> GSHMASADNNSAIYFNTSQPINDLQGSLAAEVKFAQSQILPAHPKEGDSQPHLTSLRKSLLLVRPVKADDKTPVQVEARDDNNKILGTLTLYPPSSLPDTIYHLDGVPEGGIDFTPHNGTKKIINTVAEVNKLSDASGSSIHSHLTNNALVEIHTANGRWVRDIYLPQGPDLEGKMVRFVSSAGYSSTVFYGDRKVTLSVGNTLL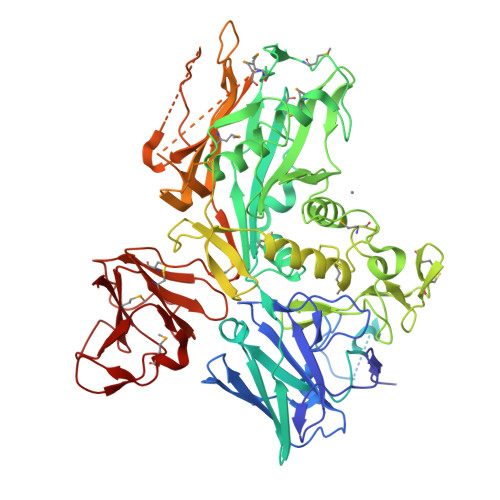FKYVNGQWFRSGELENNRITYAQHIWSAELPAHWIVPGLNLVIKQGNLSGRLNDIKIGAPGELLLHTIDIGMLTTPRDRFDFAADAAAHREYFQTIPVSRMIVNNYAPLHLKEVMLPTGELLTDMDPGNGGWHSGTMRQRIGKELVSHGIDNANYGLNSTAGLGENSHPYVVAQLAAHNSRGNYANGIQVHGGSGGGGIVTLDSTLGNEFSHDVGHNYGLGHYVDGFKGSVHRSAENNNSTWGWDGDKKRFIPNFYPSQTNEKSCLNNQCQEPFDGHKFGFDAMAGGSPFSAANRFTMYTPNSSAIIQRFFENKAVFDSRSSTGFSKWNADTQEMEPYEHTIDRAEQITASVNELSESKMAELMAEYAVVKVHMWNGNWTRNIYIPTASADNRGSILTINHEAGYNSYLFINGDEKVVSQGYKKSFVSDGQFWKERDVVDTREARKPEQFGVPVTTLVGYYDPEGTLSSYIYPAMYGAYGFTYSDDSQNLSDNDCQLQVDTKEGQLRFRLANHRANNTVMNKFHINVPTESQPTQATLVCNNKILDTKSLTPAPEGLTYTVNGQALPAKENEGCIVSVNSGKRYCLPVGQRSGYSLPDWIVGQEVYVDSGAKAKVLLSDWDNLSYNRIGEFVGNVNPADMKKVKAWNGQYLDFSKPRSMRVVYK> KDSPIIEANGTLDELTSFIGEAKHYVDEEMKGILEEIQNDIYKIMGEIGSKGKIEGISEERIAWLLKLILRYMEMVNLKSFVLPGGTLESAKLDVCRT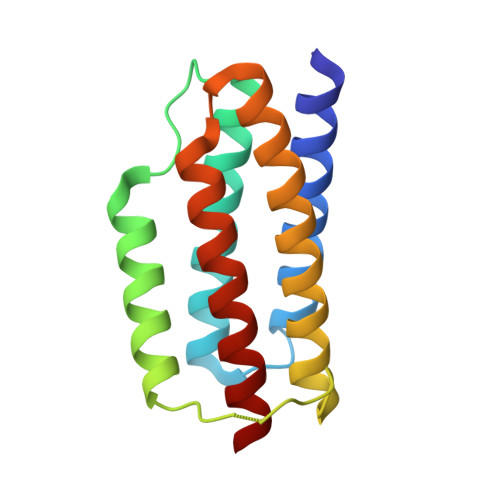IARRALRKVLTVTREFGIGAEAAAYLLALSDLLFLLARVIEIE2-methyl-1,2,3,4-tetrahydroisoquinolin-5-amine 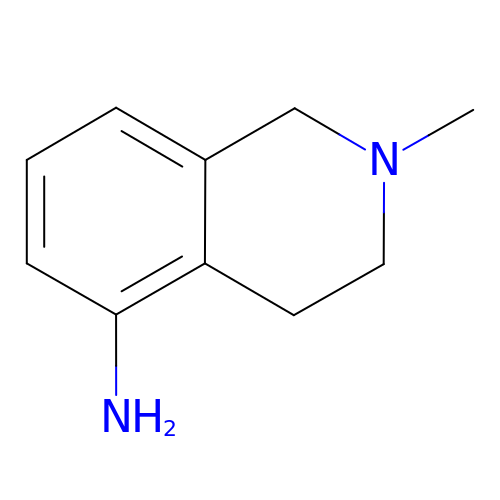| C10 H14 N2 | OXWNTTVDTPIYRD-UHFFFAOYSA-N>MAGSNDVAKVMKTLDGMREGLIQTAVELGSIEAPTGREGAAGDYVYEWMARNGFGPERVGVFDDRFNVVGRLRGTGGGASLSFNSHLDTIMAREDTARFADANDRIYHEAWHEEGRIYGYSVVNCKGPMACWLIAAKALKEAGAALKGDVVLTAVCGEIDCEPVDEFQGHDYLAEDIGARYAISHGAISDYALVAEATNFKPAWVEAGKVFLKVTVFAGPSRYTPYVPRPVAALDSPNAIVRMAKLVEALEEWADNYEKRYTREYGGGTVVPKVAIGAIRGGVPYKIYRFPELCSIYMDIRLNPDTNPLVVQREVEAVVSKLGLK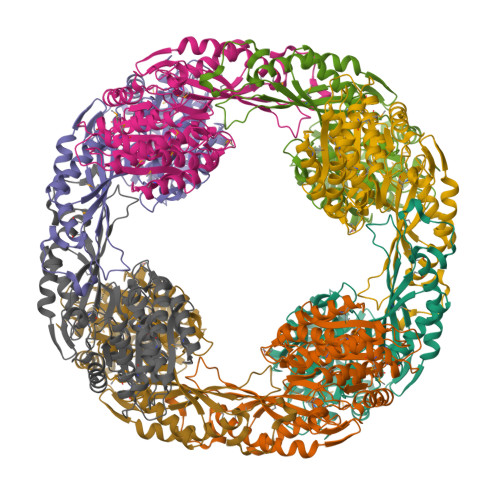AEVKPFLFRRGYEAQGIEPLQNALEVAHREVVGRPTERPGSPECSMWRDTNPYNELGIPSLTYGCGGGAGGGNTYFLVDDMLKAAKVYAMTAMDLCNRTP[4x]>SVRKILRMGDPILRKISEPVTEDEIQTKEFKKLIRDMFTTMRHAEGVGLAAPQIGILKQIVVVGSEDNERYPGTPDVPERIILNPVITPLTKDTSGFWEGCLSVPGMRGYVERPNQIRMQWMDEKGNQFDETIDGYKAIVYQHECDHLQGILYVDRLKDTKLFGFN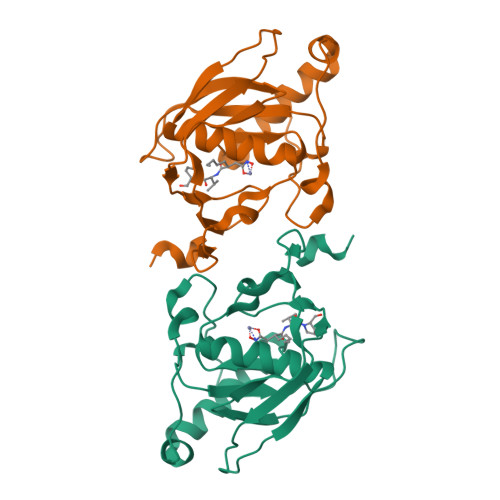ETLDSSHNVLD[8x]>MVLYFIGLGLYDERDITVKGLEIAKKCDYVFAEFYTSLMAGTTMGRIQKLIGKEIRVLSREDVELNFENIVLPLAKENDVAFLTPGDPLVATTHAELRIRAKRAGVESYVIHAPSIYSAVGITGLHIYKFGKSATVAYPEGNWFPTSYYDVIKENAERGLHTLLFLDIKAEKRMYMTANEAME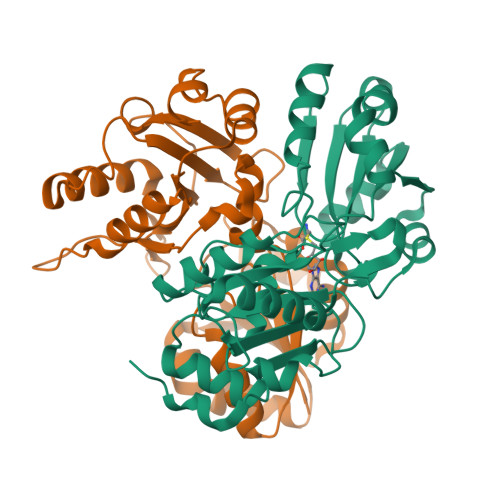LLLKVEDMKKGGVFTDDTLVVVLARAGSLNPTIRAGYVKDLIREDFGDPPHILIVPGKLHIVEAEYLVEIAGAPREILRVNV[2x]> MSLETRARNSTRPASGLIDWEQARQAALRLSQWEQAPVDNRAFRREQYARMVALSEPLIADYLGVRLPEPVSRIFVFDRREWLEANIVSFSQLFRPIEEMYEKNGGGRGALGVLMNDVSSKLLGVQIGGLLGYLAQRVLGQYDLSLLSAEATGGSLYFVEPNIARVQQQLGLSDEDFRLWITLHEMTHAFEFEAYPWVRTYFRELLEQNFALVSGQMLSSGNSLVDMLMRLLQGIGSGQHWIETVLTPEQRAVFDRIQALMSLIEGYGNHVMNAVGRRLLPSFNQIEQQIAQRQRQRTMLDQMVFRLTG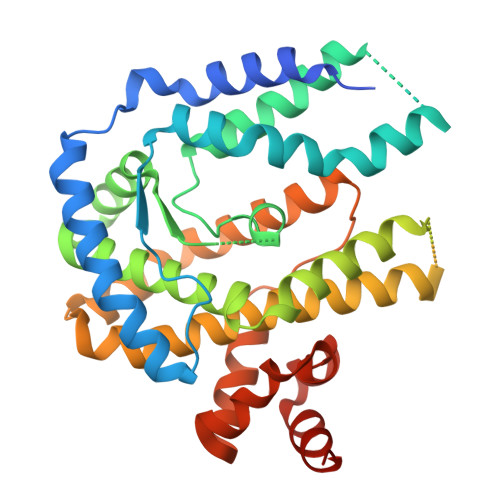LDLKLAQYQQGEAFVNAVVAARGIQFASRVWERPENLPSMDEIRNPGQWIVRMDREGHHHHHH>SNASSVTSPSSPSDVKGKSDLKDFLAIDDFDTATIKTILDKASEVKALLKSGERNYLPFKGKSMSMIFAKPSMRTRVSFETGFFLLGGHALYLGPNDIQMGKREETRDVARVLSRYNDIIMARVFAHQDILDLANYSSVPVVNGLTDHNHPCQIMADALTMIEHIGQVEGTKVVYVGDGNNMVHSWLELASVIPFHFVCACPKGYEPDKERVSKAKQAGLSKIEITNDPKEAVIGADVVYSDVWASMGQKDEAEARRKAFQGFQVDEALMKLAGQKAYFMHCLPAERGVEVTNGVVEAPYSIVFPQAENRMHAQNAIMLHLLGF[3x]

The first step of the cycle, catalyzed by ornithine transcarbamylase (ornithine carbamoyltransferase, OTC, EC 2.1.3.3), is the reaction of ornithine with carbamoyl phosphate to convert them into citrulline, with simultaneous phosphate release. AtOTC, like many other OTCs, forms a trimer, with subunits arranged around a non-crystallographic three-fold axis. The AtOTC subunit, similarly to other OTCs, is organized in two α/β domains: N-terminal (CP-binding) and C-terminal (ORN-binding) domain. The active site of AtOTC is located inside a cleft formed at the domain interface.

In the AtOTC-ORN complex, we identified additional SO4 2- ion (lithium sulfate was one of the crystallization buffer components) bound in the CP-binding location. The sulfate ion has an almost identical conformation as the phosphate moiety of CP in AtOTC-CP structure. The α-amine group of ORN creates three hydrogen bonds with side chains of N232, D293, and S297. The carboxylic group directly interacts with the N232 side chain and M298 backbone. The ϵ-amine of ORN is hydrogen-bonded with the carbonyl oxygen of L334. In the AtOTC-CP structure, where the ORN binding cleft remains empty, we were not able to trace the conformation of the SMG loop, which naturally participates in ORN binding. This region was fully structured only when ORN occupied the active site. A thorough analysis of the AtOTC-ORN structure showed that two alternative conformations of the α10 region were captured in chains A and B. The conformational changes include the SMG loop and the helix α10, namely residues 294-304. In a relaxed (open) state the loop fragment is straight and sharply turns around G299 to form a 3-turn helix α10, extending from residue K301 to A310. The loop bends, residues 301-303 move out from the helix α10 to form one turn of the 310 helix, and helix α10 significantly shifts its position.> SSDSFQRQLVQRTNTLNSSIDNATLTILSRFQDILDIAINEGKDKYTVAPEVYQIECHTVSMVRAVEQLLDVSRQIKSYWLTNSLSTSFPTVDYSEPDLEKVKRTLTKLQNHLLEVSLIEPEASETTEAPT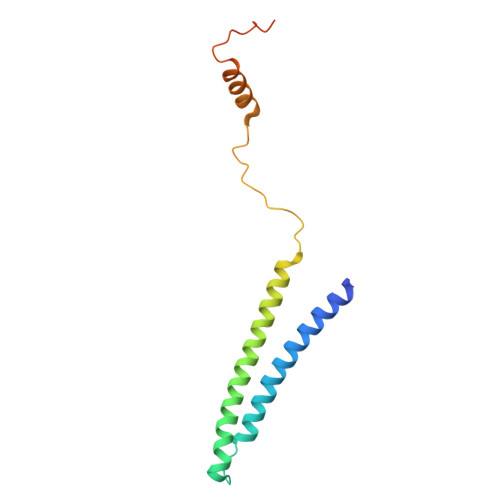VSDT>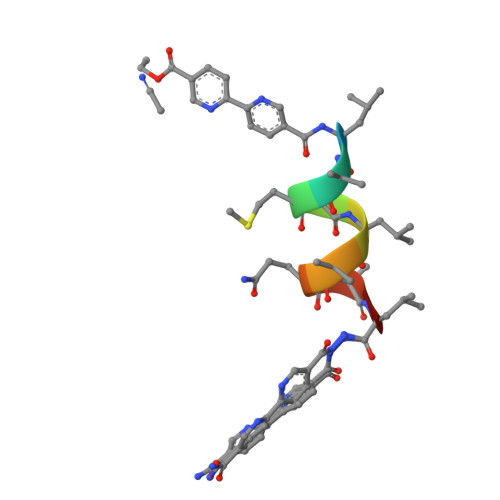XLAMALAQALX[3x]> GLKELRAVPKADIVSGFEGAKVCKDVYPKGTDPRGAVVRSTKWPNGSVITVGLYGGTPYVRSKVKQYAQEWSNYANITFNFVESGTPQIRVTFTQGAGSYSYLGTQALSIPSNEETMNFGWFDDSTSDTEFSRTVIHEFG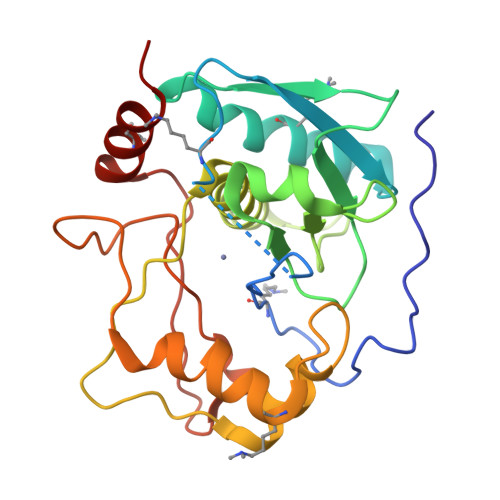HALGMIHEHQHPLTNIPWDKNKVYAYYAGYPNYWSKKDVDNNLFATYSTTQTQYSAYDTQSIMHYSISSALTTNGFSVGNNSVLSATDKQFIATVYPR> RDFNNLTKGLCTINSWHIYGKDNAVRIGEDSDVLVTREPYVSCDPDECRFYALSQGTTIRGKHSNGTIHDRSQYRALISWPLSSPPTVYNSRVECIGWSSTSCHDGKTRMSICISGPNNNASAVIWYNRRPVTEINTWARNILRTQESECVCHNGVCPVVFTDGSATGPAETRIYYFKEGKILKWEPLAGTAKHIEECSCYGERAEITCTCRDNWQGSNRPVIRIDPVAMTHTSQYICSPVLTDNPRPNDPTVGK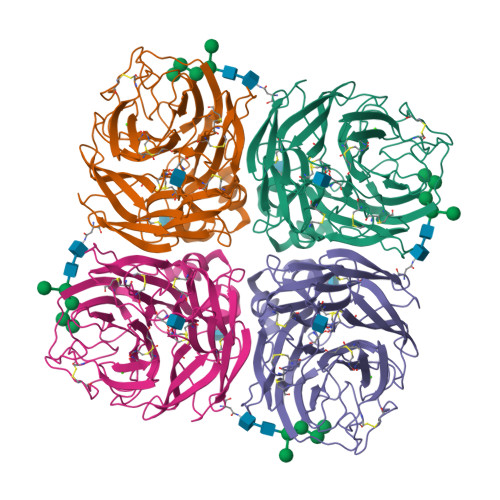CNDPYPGNNNNGVKGFSYLDGVNTWLGRTISIDSRSGYEMLKVPNALTDDKSKPTQGQTIVLNTDWSGYSGSFMDYWAEGECYRACFYVELIRGRPKEDKVWWTSNSIVSMCSSTEFLGQWDWPDGAKIEYFL~{N}-[5-(3,6-dihydro-2~{H}-pyran-4-yl)-2-methoxy-pyridin-3-yl]-2-methyl-1-(phenylmethyl)imidazole-4-sulfonamide | C22 H24 N4 O4 S | 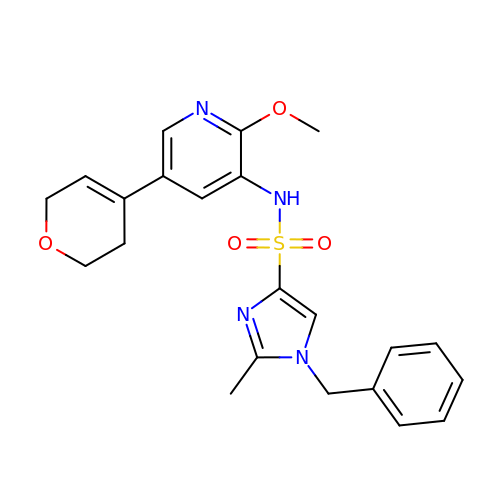HEYCQGPIBKDOSR-UHFFFAOYSA-N>[2x]ISHMSSHHHHHHIQNRAQAVDQLRAVARYFRQTEPHSPVAYLADKAAEWADMPLHKWLESVVKDDGSL

Contractile bacteriophages of the family Myoviridae (i.e. T4), R-type pyocins and the type VI secretion system (T6SS) of Gram-negative bacteria are evolutionarily related nano-scale injection machines that puncture target cell membranes using a shared contraction mechanism. TssA subunits are enigmatic as they possess a conserved N-terminal region of unknown function, previously identified as ImpA_N (PFAM: PF0681226), whereas sequences located C-terminal to this region are highly divergent. Consistent with this, phylogenetic analysis has suggested that the TssA family can be subdivided into three clades (TssA1, TssA2 and TssA3). The structural studies presented here show that TssA1B, TssA2A and TssA2B possess structurally diverse CTDs that lead to distinct overall architectures for their respective complexes.

Nested deletion of consecutive helical segments of TssA1B CTD revealed that loss of α15 resulted in the failure of the protein to assemble into a high molecular weight ring, and structure determination of the construct H12–H14 (helices α12–α14) and of that consisting of α12 and α13 alone (residues 303–347), revealed them both to be dimers. In the assembled Bc TssA1B CTD ring, analysis by PISA32 revealed an extensive dimer interface (~950 Å2) between monomers in the different layers, which principally involves the interaction of residues located in helices α12–α13 with their two-fold related subunits forming a region of hydrophobic packing with hydrophilic interactions at the periphery.AXITINIB | C22 H18 N4 O S | 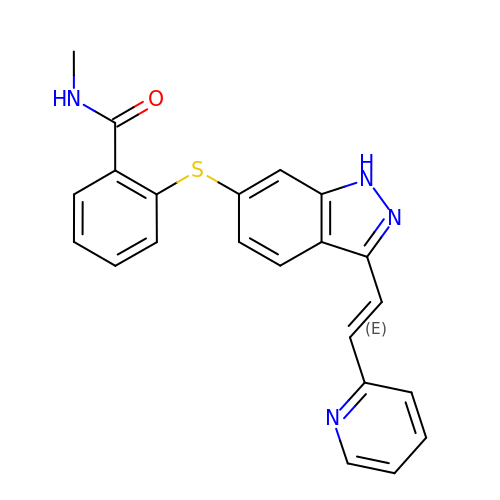RITAVMQDGBJQJZ-FMIVXFBMSA-N>MAITVSSRQLFIDGEWRVPILNKRIPNINPSTENIIGDIPAATKEDVDLAVDAAKRAISRKNGRDWSAASGSLRARYLRAIAAKIKEKKDELGKLESIDCGKPLEEALADLDDVVACFEYYAGLAEELDSKQKAPISLPMDTFKSYILKEPIGVVALITPWNYPFLMATWKIAPALAAGCAAILKPSELASVTCLELGEICKEVGLPRGVLNIVTGLGHEAGASLASHPDVDKISFTGSSATGSKIMTTAAQLVKPVSLELGGKSPIVVFEDVDLDKVAEWTVFGCFFTNGQICSATSRLIVHESIAVEFVDKLVKWAENIKISDPLEEGCRLGPIVSEAQYKKVLNCISSAKSEGATILTGGRRPEHLKKGYFVEPTIITDVTTSMQIWREEVFGPVLAVKTFSTEEEAINLANDTHYGLGSAVMSNDLERCERLSKALQAGI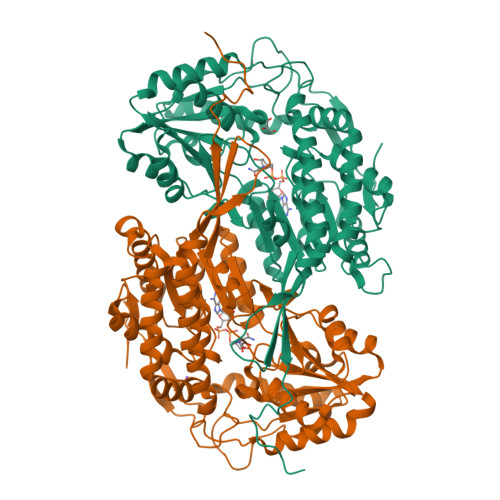VWINCAQPSFIQAPWGGIKRSGFGRELGEWGLENYLSVKQVTRYTSDEPWGWYQPPSKL[12x]>[4x]AHLLTLNEATHEVQQVKLTRDQTSYGDEIDKFWLTQYVIHRESYDFYSVQVDYTAVGLMSTPNVAESYQSKFKGRNGLDKVLGDSETTRVKINSVILDKPHGVATIRFTTVRRVRSNPVDDQPQRWIAIMGYEYKSLAMNAEQRYVNPLGFRVTSYRVNPEVN

The conjugative transfer of plasmids between Gram-negative bacteria is mediated by type IV secretion system (T4SS) and many pathogens such as Helicobacter pylori, Bartonella and Brucella species use this strategy for the transfer of virulence factors into mammalian cells. T4SS typically comprise 12 membrane-associated proteins that fall into three categories: cytoplasmic ATPases (VirB4, VirB11 and VirD4), surface-exposed pilus components (VirB2 and VirB5) and core components associated with the inner and/or the outer membrane (VirB1, VirB3, VirB6, VirB7, VirB8, VirB9 and VirB10). Here, we conducted a fragment-based screen to identify novel chemical entities that bind to and may identify novel druggable sites on TraE and other VirB8-like proteins. Also, our data demonstrate the existence of two potential druggable sites on TraE.

Using a differential scanning fluorimetry (DSF) assay in an RT-PCR instrument we screened a fragment library of 505 molecules identifying 16 molecules that significantly increase the thermal melting point of the purified periplasmic domain of TraE. Whereas docking predictions are increasingly reliable, the design of inhibitors requires high-resolution structural information and towards this goal we soaked TraE crystals with the binding fragments. Surprisingly, molecule 1E6 (2-furoic acid) bound to two sites on TraE. The first binding site is in the inhibitor-binding surface groove, whereas the second molecule binds to an α-helical region at the dimerization site of VirB8-like proteins as was predicted by docking. To our surprise, molecule 1E6 also binds to an alternative site that is close to the dimer interface of VirB8-like proteins. The discovery of this novel binding site opens additional opportunities for the design of small molecules that inhibit the functions of VirB8-like proteins. Since both fragments bind in close proximity we reasoned that combining them may generate small molecules with higher affinity. In silico docking predicted that all these molecules bind to one or both of the 1E6 binding sites observed by X-ray crystallography. Addition of the fragments as well as of the derived small molecules that do not stabilize the protein in the DSF assay at concentrations of 50 μM has no effect on conjugation.> PIPAWASGNLLTQAIR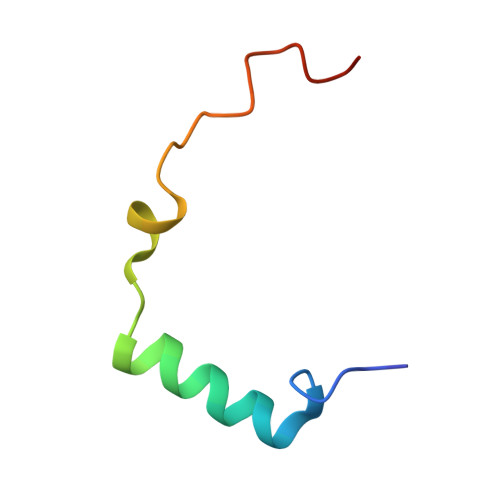QQYYKPIDVDRMYGTIDSPKLEELFNKS>[2x]MEYEWKPDEQGLQQILQLLKESQSPDTTIQRTVQQKLEQLNQYPDFNNYLIFVLTKLKSEDEPTRSLSGLILKNNVKAHFQNFPNGVTDFIK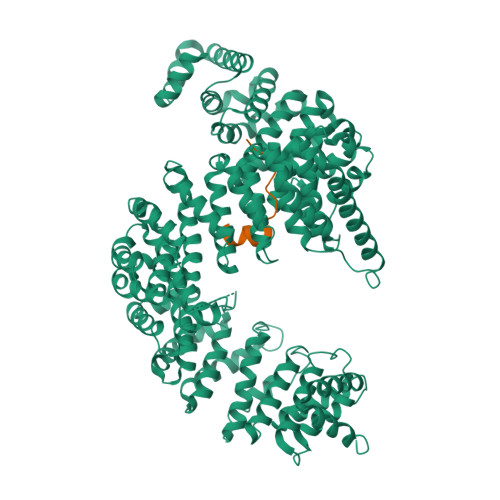SECLNNIGDSSPLIRATVGILITTIASKGELQNWPDLLPKLCSLLDSEDYNTCEGAFGALQKICEDSAEILDSDVLDRPLNIMIPKFLQFFKHSSPKIRSHAVACVNQFIISRTQALMLHIDSFIENLFALAGDEEPEVRKNVCRALVMLLEVRMDRLLPHMHNIVEYMLQRTQDQDENVALEACEFWLTLAEQPICKDVLVRHLPKLIPVLVNGMKYSDIDIILLKGDVEGGSGGSGDDTISDWNLRKCSAAALDVLANVYRDELLPHILPLLKELLFHHEWVVKESGILVLGAIAEGCMQGMIPYLPELIPHLIQCLSDKKALVRSITCWTLSRYAHWVVSQPPDTYLKPLMTELLKRILDSNKRVQEAACSAFATLEEEACTELVPYLAYILDTLVFAFSKYQHKNLLILYDAIGTLADSVGHHLNKPEYIQMLMPPLIQKWNMLKDEDKDLFPLLECLSSVATALQSGFLPYCEPVYQRCVNLVQKTLAQAMLNNAQPDQYEAPDKDFMIVALDLLSGLAEGLGGNIEQLVARSNILTLMYQCMQDKMPEVRQSSFALLGDLTKACFQHVKPCIADFMPILGTNLNPEFISVCNNATWAIGEISIQMGIEMQPYIPMVLHQLVEIINRPNTPKTLLENTAITIGRLGYVCPQEVAPMLQQFIRPWCTSLRNIRDNEEKDSAFRGICTMISVNPSGVIQDFIFFCDAVASWINPKDDLRDMFCKILHGFKNQVGDENWRRFSDQFPLPLKERLAAFYGV;>TGGKAPRKQLATKAARK[2x]>[4x]MKEEKR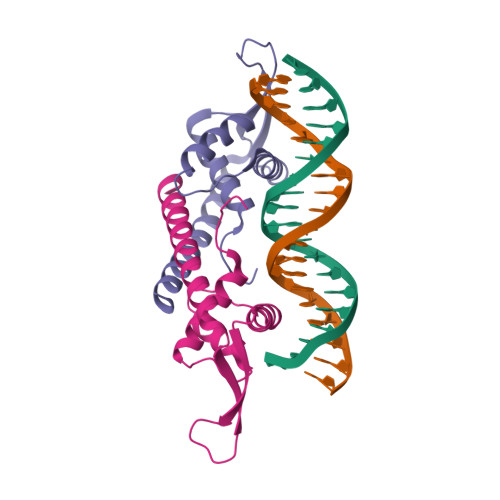SSTGFLVKQRAFLKLYMITMTEQERLYGLKLLEVLRSEFKEIGFKPNHTEVYRSLHELLDDGILKQIKVKKEGAKLQEVVLYQFKDYEAAKLYKKQLKVELDRSKKLIEKALSDNF>[2x]MASPAVRKAISDAALQYAKPEGKIFQYGTAGFRMKADLLNTVVYAVGLLATLRSKKLSGQWIGVMVTASHNPAEDNGVKLVDPMGEMLEAEWEAYATKLANAPLENIGDVYDELVKEIDVSMENPARVVFARDTRASGSRLIGVLSAALTATEAEFIDMKFMTTPQLHYVVRCKNTLGTQYEYGEPTEQGYYEKLAAAFKRVMRGVKVKGSLTVDCANGVGGPKLRELIKYLPEDTGLDIKIVNDDVINPDSLNFECGADYVKTKQRAPPSSKASILDRCASLDGDADRILYYFLDEGNVFRLLDGDRIATLAASFIGDLARSAGIAQKLKIGVVQTAYANGSSTEYIEKVLKLPSVCTNTGVKHLHHAAMRFDVGVYFEANGHGTITFSENALKTIKNTEPQSPAQQRSLECLQALTDLINQAVGDAISDMLLVEAILAHKGWTPKEWLATYTDLPSRLVRVEVAERSIFKAYDAERKLESPPGLQAKIDSLQSRYNKGRSFARASGTEDAVRVYAEAASRSEADDLATRVANAVRDAGTVKEILQAS

N-acetylphosphoglucosamine mutase (AGM1) catalyzes the interconversion of N-acetylglucosamine-6-phosphate (GlcNAc-6P) to N-acetylglucosamine-1-phosphate (GlcNAc-1P) in eukaryotes. This enzyme is a member of the α-d-phosphohexomutase superfamily of enzymes that catalyze intramolecular phosphoryl transfer on a range of phosphosugar substrates. The reaction catalyzed by AGM1 is the third step in the biosynthesis of UDP-GlcNAc from fructose-6-phosphate in the hexosamine pathway. Previously, AGM1 was shown to be an essential gene in the human fungal pathogen Aspergillus fumigatus and has been proposed as a drug target.

We also determined the crystal structure of AfAGM1 in complex with GlcNAc-6P and magnesium, showing the typical four domains forming a heart shape found previously for other members (domains 1–4). Domains 1 (residues 1–187), 2 (residues 188–305), 3 (residues 306–442), and 4 (residues 443–542) bear the predicted active serine loop, the metal-binding loop, the sugar-binding loop, and the phosphate-binding, respectively. At the active site of one of the two monomers in the asymmetric unit, unambiguous electron density defining a phosphorylated Ser (Ser69) was present. The conformation of the phosphoserine with an O…..P–O angle of 158° would facilitate inline attack/displacement by the GlcNAc-6P O1 and hence further supports the role of this residue as the phosphoryl donor/acceptor. The dephospho-AfAGM1–GlcNAc-6P complex has an overall structure with an open active site and may represent the inactive enzyme or ‘apo’ like conformation. This complex provides the likely snapshot of the conformation of the protein just before the first phosphoryl transfer or the release of product from the active site. The phospho-AfAGM1–GlcNAc-6P–Mg2+ Michaelis complex reveals a semi-opened active site and may represent the active complex. For this complex, it was observed that GlcNAc-6P made hydrogen bond interactions with residues R505, R514, S507, T509, G508, E380 and V363 from domains 3 and 4 of the protein but not with any residues from domains 1 and 2. Furthermore, the AfAGM1_pSer69 establishes hydrogen bond interactions with residues R33, R289 and H70 from domains 1 and 2 as well as Mg2+, which is co-ordinated by D288, D284 and D286; hence, domains 3 and 4 relax to open the active site cleft. In AfAGM1, the magnesium ion is pentagonally co-ordinated in a square pyramidal arrangement by AfAGM1_pSer69, Asp284, Asp286, and Asp288.>GQLSVDNGLWRVTLCMLAFPLLLTGLISFREKRLQDVGTPAARARAFFTAPVVVFHLNILSYFAFLCLFAYVLMVDFQPVPSWCECAIYLWLFSLVCEEMRQLFYDPDECGLMKKAALYFSDFWNKLDVGAILLFVAGLTCRLIPATLYPGRVILSLDFILFCLRLMHIFTISKTLGPKIIIVKRMMKDVFFFLFLLAVWVVSFGVAKQAILIHNERRVDWLFRGAVYHSYLTIFGQIPGYIDGVNFNPEHCSPNGTDPYKPKCPESDATQQRPAFPEWLTVLLLCLYLLFTNILLLNLLIAMFNYTFQQVQEHTDQI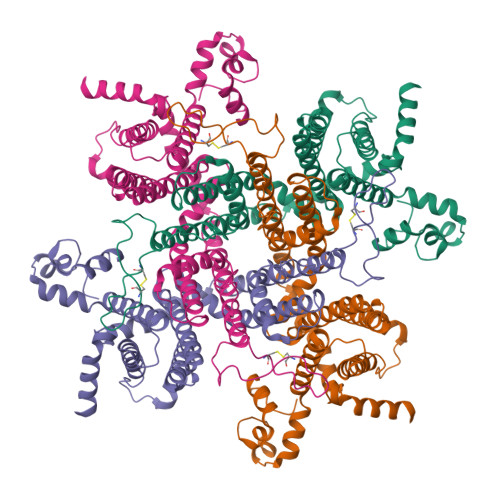WKFQRHDLIEEYHGRPAAPPPFILLSHLQLFIKRVV[4x]> GSHMNVDLVFLFDGSMSLQPDEFQKILDFMKDVMKKLSNTSYQFAAVQFSTSYKTEFDFSDYVKRKDPDALLKHVKHMLLLTN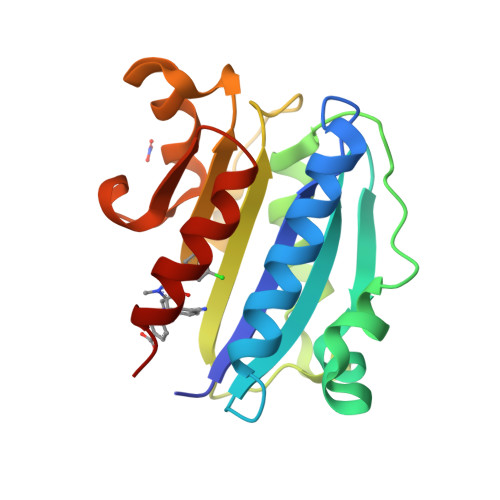TFGAINYVATEVFREELGARPDATKVLIIITDGEATDSGNIDAAKDIIRYIIGIGKHFQTKESQETLHKFASKPASEFVKILDTFEKLKDLFTELQKKIY>HHHHHHMAGEKSTIIYTLTDEAPLLATYSLLPIIETFTKPAGIEIVKSDISVAARVLAEFADYLSEEQKVSDNLAELGRLTQDPDTNIIKLPNISASVAQLTACIKELQSKGYAIPDYPENPATEEEKTIKARYGKCLGSAVNPVLREGNSDRRAPAAVKNYAKKHPHSMSEWKQWSQTHVSHMEEGDFYHGEKSMTLDRPRNVKMELITNSGKSIVLKPKVALQEGEIIDSMFMSKKALCDFYEKQLDDCREAGILFSLHVKATMMKVSHPIVFGHCVKIYYKEAFEKHGKLFDELGINVNNGMAGLYEKIETLPTSLREEIIEDLHACQEHRPALAMVDSAKGITNFHSPNDIIVDASMPAMIRAGGKMWGADGKQYDAKAVMPESTFARIYQEMINFCKWHGNFDPKTMGTVPNVGLMAQKAEEYGSHDKTFEIPEAGIANITDLDTGEVLLTQNVEEGDIWRMCQVKDAPIRDWVKLAVTRARNSGMPAIFWLDPYRPHENELIKKVQKYLKDHDTTGLDIQIMSQVRAMRYTLERVVR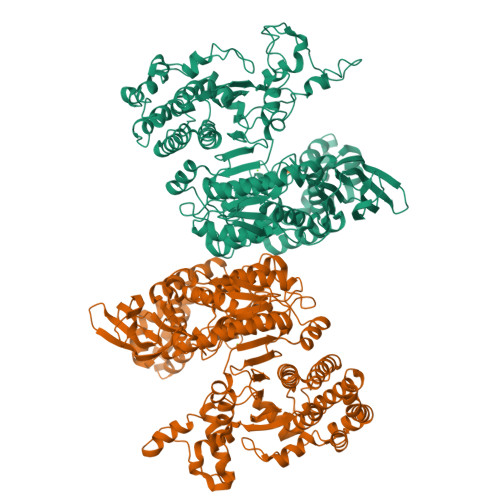GLDTISVTGNILRDYLTDLFPIMELGTSAKMLSIVPLMAGGGMYETGAGGSAPKHVQQLVEENHLRWDSLGEFLALAVSLEEMGIKENNARTKLLAKTLDEATGKLLDNDKSPSRRTGELDNRGSHFYLSLYWAEALAAQNEDAELKAKFAPLAKALAENEQKIVAELAQVQGKPADIGGYYAVDPAKVSAVMRPSATFNAALSTVQA[2x]> MGSSHHHHHHGSNQLTAYTLRLGDNCLVLSQRLGEWCGHAPELEIDLALANIGLDLLGQARNFLSYAAELAGEGDEDTLAFTRDERQFSNLLLVEQPNGNFADTIARQYFIDAWHVALFTRLMESRDPQLAAISAKAIKEARYHLRFSRGWLERLGNGTDVSGQKMQQAINKLW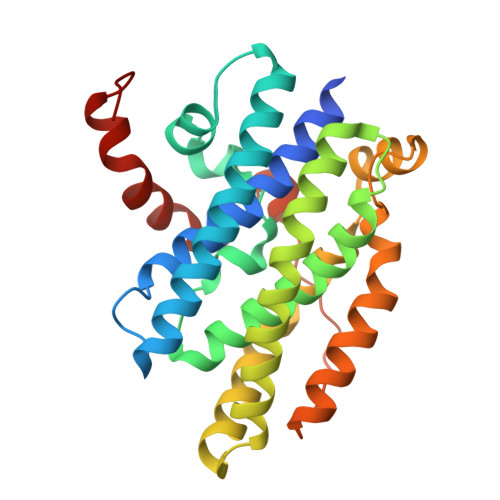RFTAELFDADEIDIALSEEGIAVDPRTLRAAWEAEVFAGINEATLNVPQEQAYRTGGKKGLHTEHLGPMLAEMQYLQRVLPGQQW> DLPKFGELLQNVTVPVSREAVLQCVVDNLQTYKIAWLRVDTQTILTIQNHVITKNHRMSITHAEKRAWILRIRDVKESDKGWYMCQINTDPMKSQVGYLDVVVPPDILDYPTSTDMVIREGSNVTLKCAATGSPTPTITWRREGGELIPLPNGAEAVAYNGSFLTIAKVNRLNMGAYLCIASNGIPPTVSKRVMLIVHFPPMIWIQNQLVGAALTQNITLECQSEAYPKSINYWMKNDTIIVPGERFVPETFESGYKITMRLTIY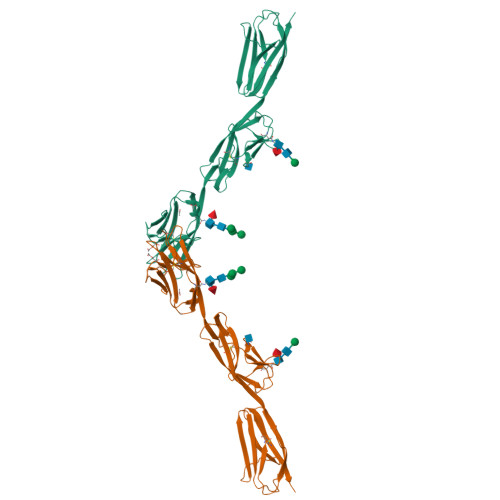EVDIQDFGAYRCVAKNSLGDTDGAIKLYHIPHHHHHH>[5x]MNRRVLVTGATGLLGRAVHKEFQQNNWHAVGCGFRRARPKFEQVNLLDSNAVHHIIHDFQPHVIVHCAAERRPDVVENQPDAASQLNVDASGNLAKEAAAVGAFLIYISSDYVFDGTNPPYREEDIPAPLNLYGKTKLDGEKAVLENNLGAAVLRIPILYGEVEKLEESAVTVMFDKVQFSNKSANMDHWQQRFPTHVKDVATVCRQLAEKRMLDPSIKGTFHWSGNEQMTKYEMACAIADAFNLPSSHLRPITDSPVLGAQRPRNAQLDCSKLETLGIGQRTPFRIGIKESLWPFLIDKRWRQTVFHAENLYFQ

MAT (methionine adenosyltransferase, also known as S-adenosylmethionine synthetase; EC 2.5.1.6) is the only known enzyme that synthesizes SAM (S-adenosylmethionine), the principle methyl group donor and precursor for polyamine and glutathione synthesis. The function of MAT2A is further dependent upon an interaction with the auxiliary subunit MAT2B, encoded by the MAT2B gene. MAT2B is present only in mammals and bears no sequence homology with the catalytic MAT1A/2A subunits, but instead harbours signature motifs of the SDR (short-chain dehydrogenase/reductase) superfamily. MAT2B was proposed to modulate the catalytic activity of MAT2A by lowering its Km value for its substrate Met and the Ki value for its product SAM.

We subsequently co-crystallized hMAT2B with NADP and resveratrol and determined the ligand-bound structure (hMAT2Bresv) at 2.8 Å resolution. Minor structural variations between the two structures are found in a loop region of the second domain (residues 282–289, loop C), forming an extended coil in the hMAT2Bresv structure and a two-turn helix in the MAT2Bsubt structure. Each hMAT2Bresv protomer is bound with an NADP molecule in its extended configuration, packing against backbone atoms from the conserved GxxGxxG motif. In the case of hMAT2B, the preference for NADP over NAD can be explained by Gly59, which provides the space to accommodate the phosphate moiety, and Arg62, which forms hydrogen bonds to the phosphate oxygens. The MAT2Bresv structure reveals two bound resveratrol molecules (res1 and res2) per protomer, which exhibit different binding modes to the protein (spheres). Res1 is positioned at the interdomain cleft of each monomer, in a putative ‘active site’ where most SDR enzymes bind their cognate substrates. The benzene-1,3-diol group of res1 forms aromatic stacking with the NADP nicotinamide ring and the diol oxygens form hydrogen bonds with Ser136, Asp137, Tyr159 and Arg219. Res2 slots into a narrow pocket that is formed by the C-terminal residues of one protomer (A), as well as the loop L1–helix α2 region of the adjacent NCS (non-crystallographic symmetry)-related protomer (B) within the asymmetric unit. Res2 is positioned within the hMAT2Bresv dimer interface mainly by van der Waals contacts and hydrogen bonds with two acidic residues (Glu68 and Asp84). The hMAT2Bresv structure did reveal a head-to-tail dimeric packing for the two NCS-related protomers within the asymmetric unit, but it probably represents a crystallization artefact for the following reasons: (i) the C-terminus involved at the interface is partly derived from the vector-encoded sequence (AENL; residues 335–338), (ii) no equivalent dimerization is observed in the hMAT2Bsubt crystal lattice, and (iii) size-exclusion chromatography of full-length hMAT2B does not reveal a dimeric species in solution.The ferric iron uptake (Fiu) transporter is a TBDT responsible for import of molecules containing the catecholate functional group. Members of the TonB-dependent transporter (TBDT)3 family drive transport of their substrates through interaction with the energy-transducing protein TonB. The structure of Fiu consists of a 22-stranded transmembrane β-barrel characteristic of the TBDT superfamily, with a number of extended extracellular loops that might serve in the initial steps of substrate binding. In addition to its role in iron uptake, Fiu has also been shown to be important for sensitivity to antimicrobials that share the common feature of a catecholate functional group or the analogous dihydroxypyridine moiety.

The structure of Fiu was solved in three different crystal forms, revealing Fiu in two distinct states. In contrast, in crystal state 2, the entire polypeptide chain (amino acids 50–760) C-terminal of the TonB box (which is disordered in both crystal forms) could be modeled into the available electron density. The disorder of the plug domain loop in crystal state 1 opens a large cavity in the interior of Fiu to the external environment, whereas, in crystal state 2, this cavity is present but occluded in the lumen of the Fiu barrel. In crystal state 2, removal of the labile subdomain opens the internal cavity of Fiu to the periplasm, but because of the presence of the plug loop, this does not create a membrane-spanning channel. For the first run, the entire extracellular portion of closed Fiu (crystal state 2) was defined as the search area. In this experiment, the majority of the solutions placed Fe–DHB in the internal chamber of Fiu, with the third most favored solution positioning Fe–DHB in the extracellular cavity of the protein. Although the internal cavity would be inaccessible to Fe–DHB in the closed state, because of the fully ordered plug loop, it would be accessible in state 1, as this loop is disordered. Specifically, the external plug loop of Fiu in our structures selectively gates a large cavity in the lumen of the transporter.

>AEGQTNADDTLVVEASTPSLYAPQQSADPKFSRPVADTTRTMTVISEQVIKDQGATNLTDALKNVPGVGAFFAGENGNSTTGDAIYMRGADTSNSIYIDGIRDIGSVSRDTFNTEQVEVIKGPSGTDYGRSAPTGSINMISKQPRNDSGIDASASIGSAWFRRGTLDVNQVIGDTTAVRLNVMGEKTHDAGRDKVKNERYGVAPSVAFGLGTANRLYLNYLHVTQHNTPDGGIPTIGLPGYSAPSAGTAALNHSGKVDTHNFYGTDSDYDDSTTDTATMRFEHDINDNTTIRNTTRWSRVKQDYLMTAIMGGASNITQPTSDVNSWTWSRTANTKDVSNKILTNQTNLTSTFYTGSIGHDVSTGVEFTRETQTNYGVNPVTLPAVNIYHPDSSIHPGGLTRNGANANGQTDTFAIYAFDTLQITRDFELNGGIRLDNYHTEYDSATACGGSGRGAITCPTGVAKGSPVTTVDTAKSGNLMNWKAGALYHLTENGNVYINYAVSQQPPGGNNFALAQSGSGNSANRTDFKPQKANTSEIGTKWQVLDKRLLLTAALFRTDIENEVEQNDDGTYSQYGKKRVEGYEISVAGNITPAWQVIGGYTQQKATIKNGKDVAQDGSSSLPYTPEHAFTLWSQYQATDDISVGAGARYIGSMHKGSDGAVGTPAFTEGYWVADAKLGYRVNRNLDFQLNVYNLFDTDYVASINKSGYRYHPGEPRTFLLTANMHF[4x]> MGVEAAKKEIKKLKEEVLKKYKKG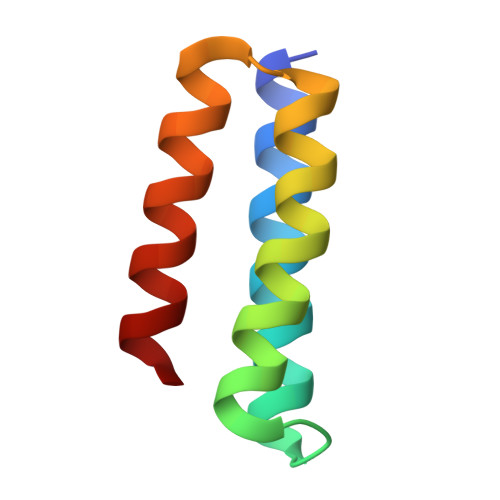EINEEEAIKEFVEKALKLVKAVGDEAVKKFAIEEAKALVEEL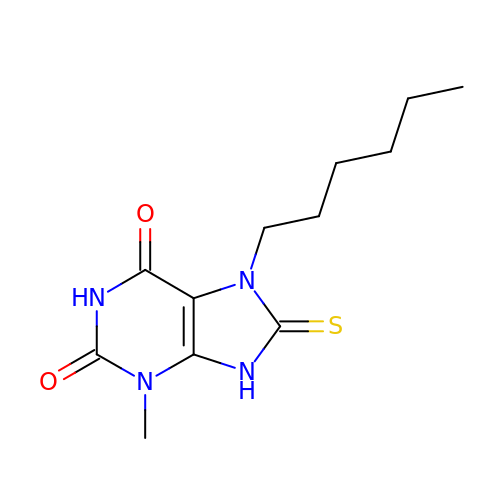7-hexyl-3-methyl-8-sulfanylidene-9H-purine-2,6-dione | C12 H18 N4 O2 S | UXIHCIYDMGYKSF-UHFFFAOYSA-N>PTIHDHRYRCLVQLLTKLRKEASLSQSELAIFLGLSQSDISKIESFERRLDALELFELLEVVASRLG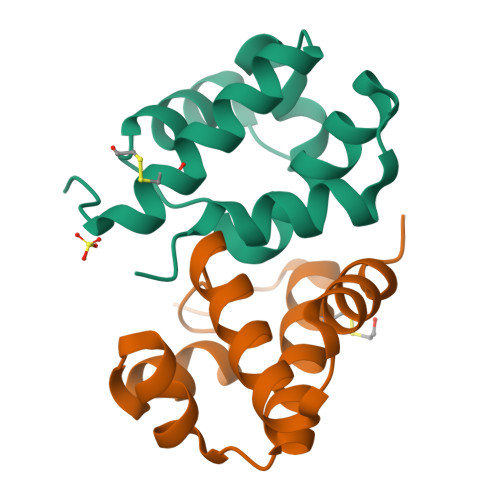LPMDILLKDTYESISKS[2x]> GGLEKDFLPLYFGWFLTKKSSETLRKAGQVFLEELGNHKAFKKELRHFISGDEPKEKLELVSYFGKRPPGVLHCTTKLCDYGKAAGAEEYAQQEVVKRSYGKAFKLSISALFVTPKTAGAQVVLTDQELQLWPSDLDKPSASEGLPPGSRAHVTLGCAADVQPVQTGLDLLDILQQVKGGSQGEA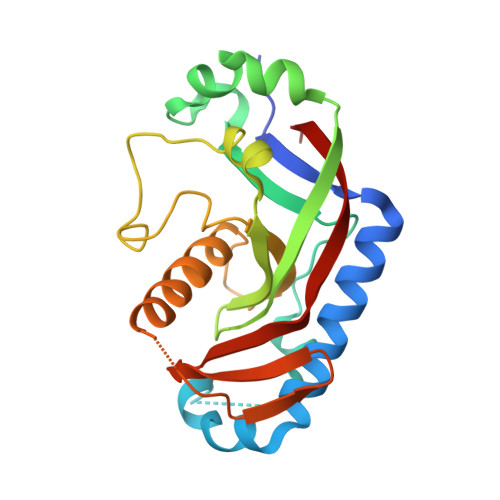VGELPRGKLYSLGKGRWMLSLTKKMEVKAIFTGYYG> EVIDTTLKATVVTKKADLIELDAADNGDALAKLLANLDIKDQNGNPMVDSAATPNTNEKLQALKSVLSGIVSSDTSVIGSVSNVDNLKDDASISGLAVKKAGTVTLTLVFNEDSKIAPIAITVKAPAATQDGVTVTGLDLVPGVTGVGKTKFTATDKIKSGHKLYYAVDDSAVPAPAVGTTRNSTKFANEITVGTTEVAANAGQIITVIEVDSSDRVVGYKTFTVE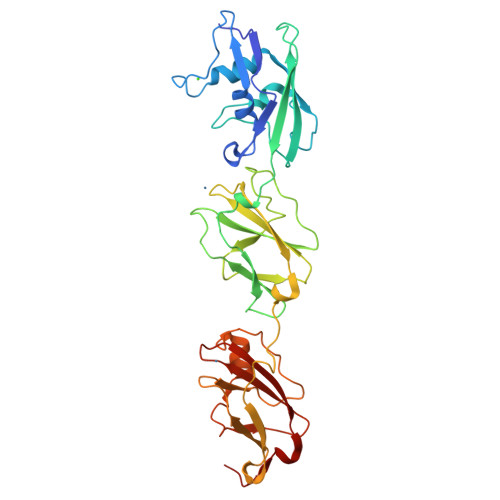AADLSVAADKTGFTATVTPTGGNQVTTGKTLLAVSDLANGHKLYAAAAGSSAAAAPVKGIAYTDTTVRTTYGTEVTSGTVEVDAQDGQHISIIEVDENGKVVGYKDYTITGIQIGTKSAS>[2x]HWSQAALYAEVQQHQARQMHALDEGKFEEYAD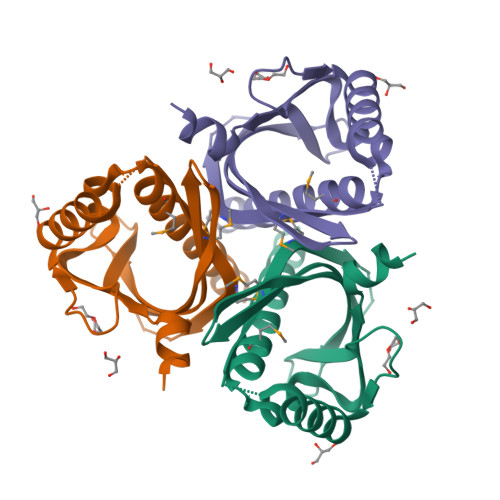TFTPDGVFRHTPGRDPAIGREAIVRELNEFHERYAEDPVQRRHMFTMLAIDELDELDDSAVQADFYTLVLTTRVDGLTVGPSCPVRDVLVRGADGRLLTASRWVEHDNRTVAE>GSHMPMYEVQWKVVEESNGNNYSYIDPTQLPYDHKWEFPRNRLSFGKTLGAGAFGKVVEATAQGLIKSDAAMTVAVKMLKPSAHSTEREALMSELKVLSYLGNHENIVNLLGACTHGGPTLVITEYCCYGDLLNFLRRKRDEFVPYKVAPEDLYKDFLTLEHLLSFSYQVAKGMAFLASKNCIHRDLAARNILLTHGNITKICDFGLARDIKNDSNYVDKGNARLPVKWMAPESIFNSVYTFESDVWSYGIFLWELFSLGSSPYPGMPVD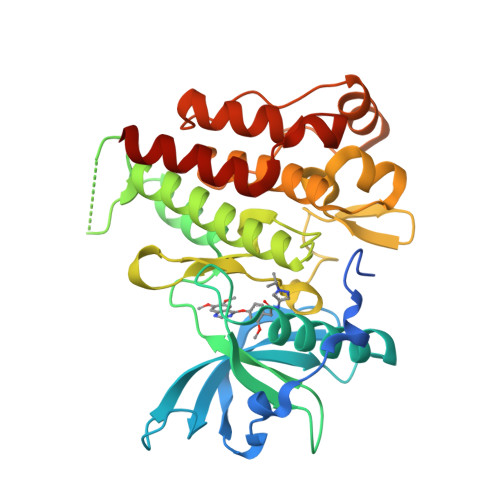SKFYKMIKEGFRMSSPEYAPAEMYDIMKTCWDADPDKRPTFKQIVQDIEKQISESTN[2x]>GTSPIQTPINTMSQQYTLPPLPYPYDALQPYISQQIMELHHKKHHQTYVNGLNAALEAQKKAAEATDVPKLVSVQQAIKFNGGGHINHSLFWKNLAPEKSGGGKIDQAPVLKAAIEQRWGSFDKFKDAFNTTLLGIQGSGWGWLVTDGPKGKLDITTTHDQDPVTGAAPVFGVDMWEHAYYLQYLNDKASYAKGIWNVINWAEAENRYIAG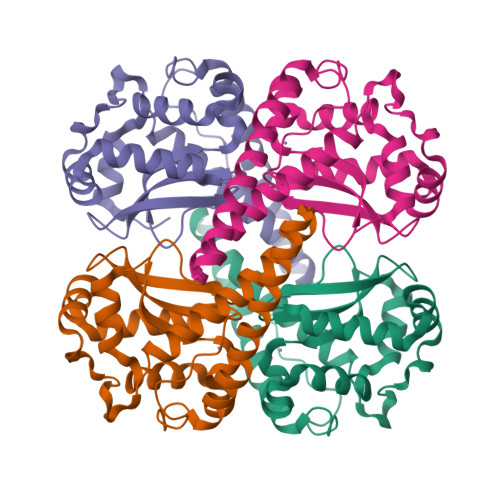DKGGHPFMKL[4x]>[2x]MRASFLLTAGLATAAVGRAKSVPKKFPFKPENSKTTGTNAIPIVYGLSESQPNSVGGSWWSSSYITTTNNEQYVVLAHYLDNPVYTYFRASTLNLETNEYHQYVTVGSSTPNITTLDVSVGNNGIKSESEDNLSKLRSYSNHDNVTFDITYDATTGAVANGGAGTFQFGEGLT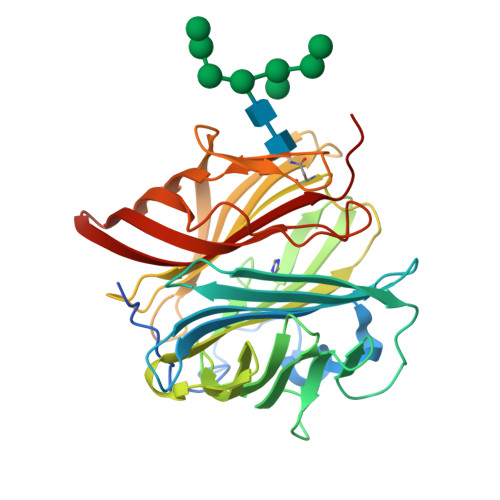WEFGLPSAKTEGSLTVHGEKLAIDPAKSHTWYDRQWGNTAAIPSNWTWFQLHIPSTEYKISAWIFSDPFRNTETRFATIRGANDETLVLPLEFTPIYKRTYESATGRVTYPLDWKLKISGFGDFKLSSYTEDQELVGEDALQTAYEGFITFSGNVHSKPVQGYGLVEIVYSTWDV>[3x]MRGSHHHHHHGLVPRGSIPALDYNPWEAIQLPTTATILDMSFIDRHHGWLVGVNATLMETRDGGQTWEPRTLVLDHSDYRFNSVSFQGNEGWIVGEPPIMLHTTDGGQSWSQIPLDPKLPGSPRLIKALGNGSAEMIT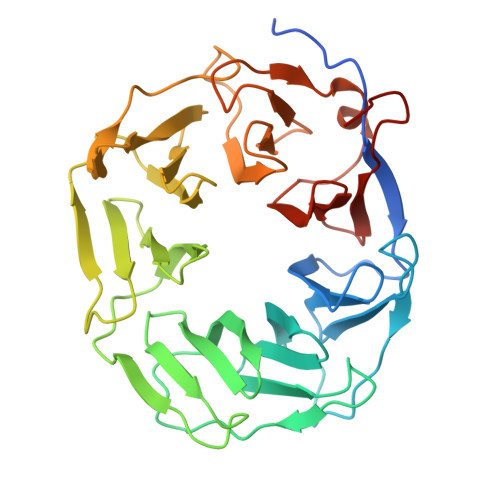NVGAIYRTKDSGKNWQALVQEAIGVMRNLNRSPSGEYVAVSSEGSFYSTWEPGQTAWEPHNETTSEELHNMGFTPDGRLWMIVNGGKIAFSDPDNSENWGELLSPLRRNSVGFLDLAYRTPNEVWLAGGAGALLCSQDGGQTWQQDVDVKKVPSNFYKILFFSPDQGFILGQKGILLRYVTDLTAAPA>SMQDTDNQAKIIPKPTPTPLSLESGMKGENWRKIEPENIVVITTKYGDILIELNPEFAPGHVARFQDMVKARAYNGKEFYRVIDGFVAQGGIDAEDKKWPPLEIEHEQPLLEADQIQLLDNDDLFAEKVGFLNGFPVGFDAEKKWLLHCPGMLAMARDSDPNTGGTDFYITLDAQRYLDRNMTVFGRVISGMQYVQKLQRGDKNIEGGVIQSPNKGDEMISVKLASELPENQQPNYEVMRTETAGFMNSINSKRVRS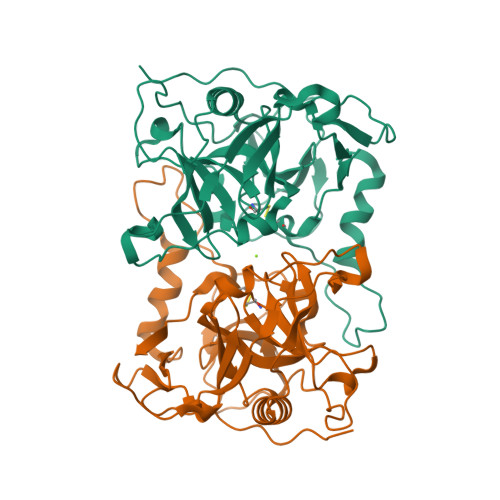DPFFFNTPPQVVDVCDVEVPTELVDF[6x]>[2x]NQCPTDWEAEGDHCYRFFNTLTTWENAHHECVSYSCSTL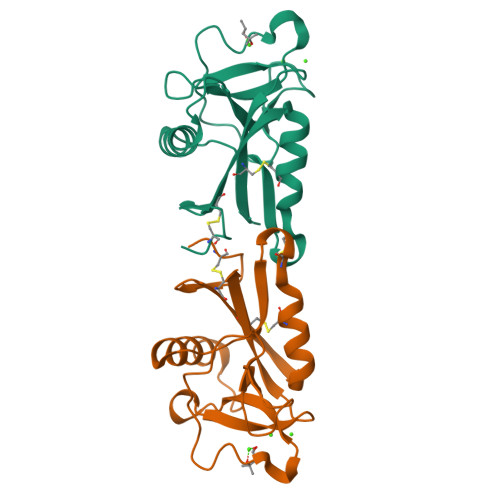NVRSDLVSVHSAAEQAYVFNYWRGIDSQAGQLWIGLYDKYNEGDFIWTDGSKVGYTKWAGGQPDNWNNAEDYGQFRHTEGGAWNDNSAAAQAKYMCKLTFE N-[6,6-dimethyl-5-[(2S)-4-methyl-2-(phenylmethyl)piperazin-1-yl]carbonyl-2,4-dihydropyrrolo[3,4-c]pyrazol-3-yl]-3-phenoxy-benzamide 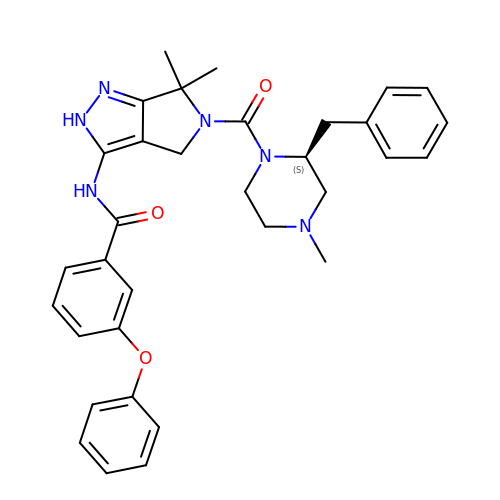| C33 H36 N6 O3 | VGRHRLOVUZTBHT-VWLOTQADSA-N>GPGYQDPMAKNIQAIRGMNDYLPGETAIWQRIEGTLKNVLGSYGYSEIRLPIVEQTPLFKRAIGEVTDVVEKEMYTFEDRNGDSLTLRPEGTAGCVRAGIEHGLLYNQEQRLWYIGPMFRHERPQKGRYRQFHQLGCEVFGLQGPDIDAELIMLTARWWRALGISEHVTLELNSIGSLEARANYRDALVAFLEQHKEKLDEDCKRRMYTNPLRVLDSKNPEVQALLNDAPALGDYLDEESREHFAGLCKLLESAGIAYTVNQRLVRGLDYYNRTVFEW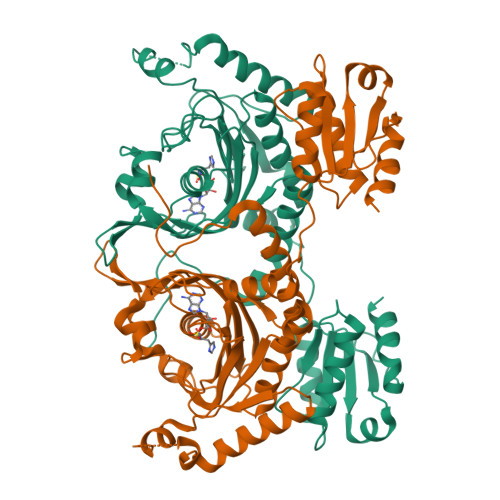VTNSLGSQGTVCAGGRYDGLVEQLGGRATPAVGFAMGLERLVLLVQAVNPEFKADPVVDIYLVASGADTQSAAMALAERLRDELPGVKLMTNHGGGNFKKQFARADKWGARVAVVLGESEVANGTAVVKDLRSGEQTAVAQDSVAAHLRTLLG[4x]>[6x]GPGSRAGAAEEPGVRGLLASLFAFKSFRENWQRAWVR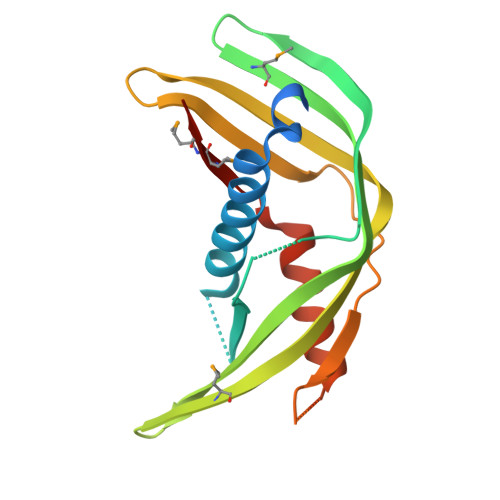ALNEQACRNGSSIQIAFEEVPQLPPRASISHVTCVDQSEHTMVLRCQLSAEEVRFPVSVTQQSPAAVSMETYHVTLTLPPTQLEVNLEEIPGEGLLISWAFTDRPDLSLTVLPKLQARERGEEQVELSTIEELIKDAIVSTQPAMMVNLRAC N-benzyl-1-{2-chloro-5-[2-(2-chloro-5-{5-(methylsulfonyl)-1-[3-(morpholin-4-yl)propyl]-4,5,6,7-tetrahydro-1H-pyrazolo[4,3-c]pyridin-3-yl}phenyl)ethyl]phenyl}methanamine 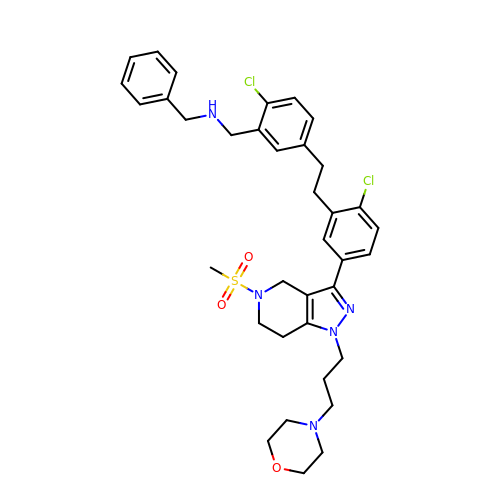| C36 H43 Cl2 N5 O3 S | ZWXXUSFMMWHRMT-UHFFFAOYSA-N methyl 1-[(2,6-dichlorophenyl)methyl]-1H-pyrazole-3-carboxylate | C12 H10 Cl2 N2 O2 | 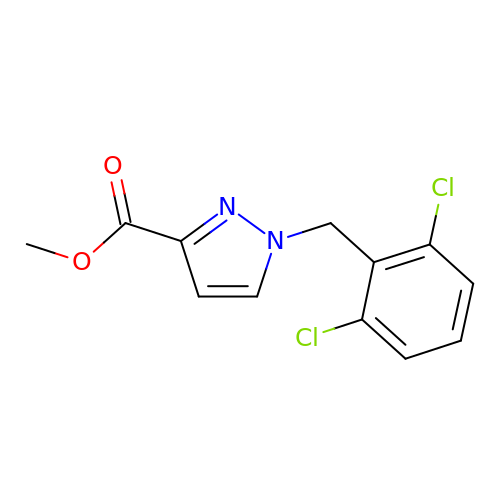CLGZXCPIPUTMMX-UHFFFAOYSA-N>[2x]TDKERFIASLMARMSNAEKIGQLRLVSVGADHPKEALMADIRAGKVGAIFNTVTRPDIRAMQDQVRHSRLKIPLFHAYDV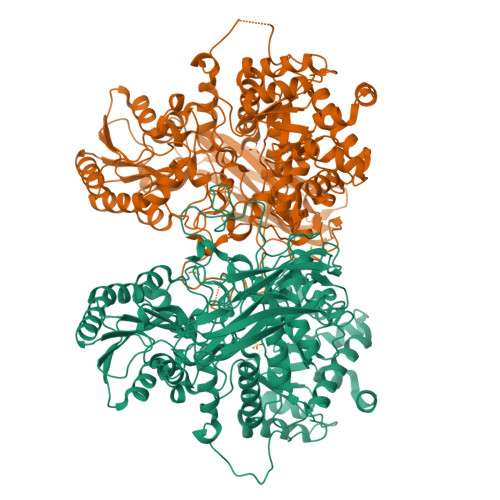AHGHRTIFPISLGLAASWDPEVVARSARISALEASADGLDMSFSPMVDITRDARWGRVSEGFGEDTYLTSLLSGVMVRAYQGSNLAAPDSIMAAVKHFALYGAAEGGRDYNTVDMSLPRMFQDYLPPYKAAVDAGAGAVMVSLNTINGVPATANRWLLTDLLRQQWGFKGLTISDHGAVKELIKHGLAGNERDATRLAIQAGVDMNMNDDLYSTWLPKLLAAGEIDQADIDRACRDVLAAKYDLGLFADPYRRLGKPDDPPFDTNAESRLHRQAAREVAREGLVLLKNRDGLLPLKKQGRIAVIGPLAKSQRDVIGSWSAAGVPRQAVTVYQGLANAVGERATLLYAKGANVSGDQAILDYLNSYNPEVEVDPRSAEAMLEEALRTARDADLVVAVVGESQGMAHEASSRTDLRIPASQRRLLKALKATGKPLVLVLMNGRPLSLGWEQENADAILETWFSGTEGGNAIADVLFGEHNPSGKLTMSFPRSVGQVPVYYNHLNTGRPMDHDNPGKYTSRYFDEANGPLYPFGYGLSYTEFSLSPLRLSSERLARGATLEARVTLSNSGKRAGATVVQLYLQDPVASLSRPVKELRGFRKVMLEPGESREIVFRLGEADLKFYDSQLRHTAEPGEFKVFVGLDSAQTESRSFTLL>MVMKILQILSRLYVADLNPALEFYEELLETPVAMRFEIPQTGVELAQISTILLIAGSEEALKPFRNTQATFLVDSLDKFKTFLEENGAEIIRGPSKVPTGRNMTVRHSDGSVIEYVEHSKIEAENLYFQSHHHHH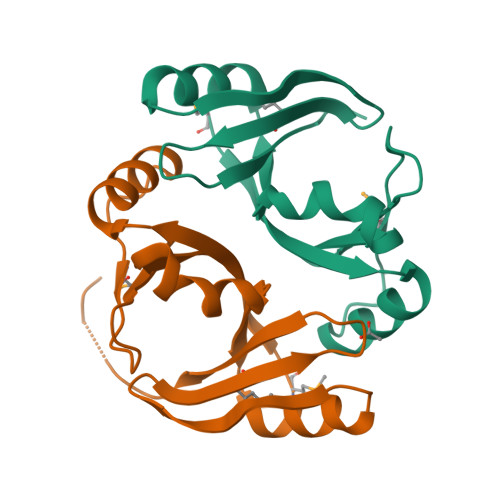HWSHPQFEK[2x]>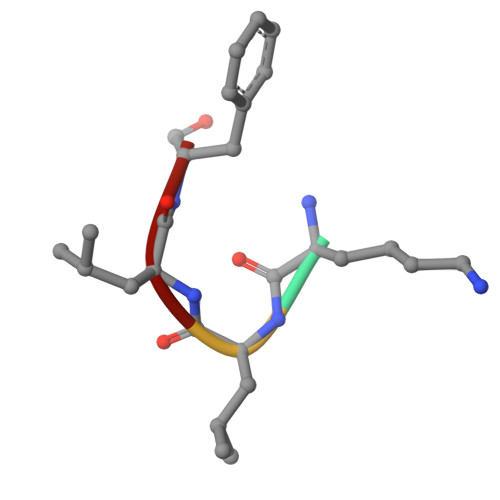 KLLF pentalenolactone F | C15 H18 O5 | 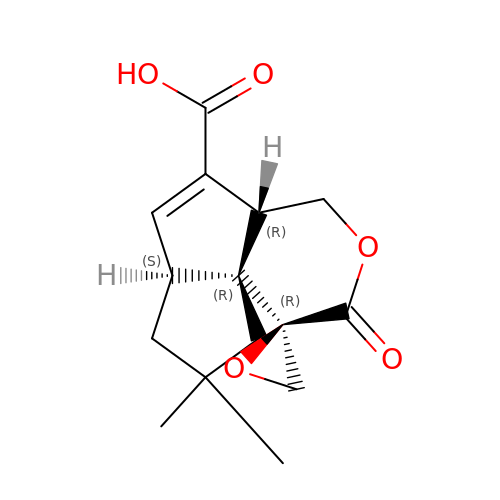UUDKOVSZNMZKND-BDAURDKOSA-N> MVNRIE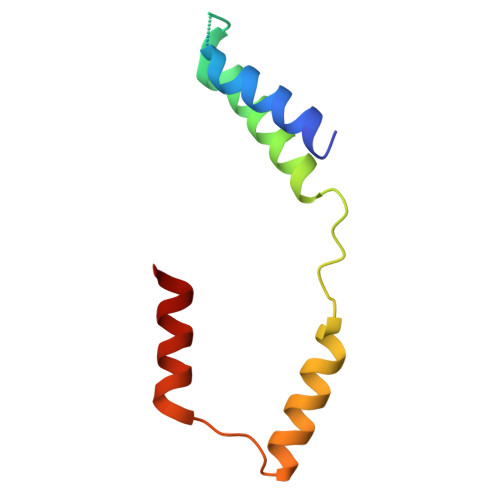LSRLIGLLLETEKRKNTEQKESGTNKIEDKVTLSKIAQELSKNDVEEKDLEKKVKELKEKIEKGEYEVSDEKVVKGLIEFFT>MTAQISPTVVDAVVIGAGFGGIYAVHKLHNEQGLTVVGFDKADGPGGTWYWNRYPGALSDTESHLYRFSFDRDLLQDGTWKTTYITQPEILEYLESVVDRFDLRRHFRFGTEVTSAIYLEDENLWEVSTDKGEVYRAKYVVNAVGLLSAINFPDLPGLDTFEGETIHTAAWPEGKNLAGKRVGVIGTGSTGQQVITALAPEVEHLTVFVRTPQYSVPVGNRPVTKEQIDAIKADYDGIWDSVKKSAVAAGFEESTLPAMSVSEEERNRIFQEAWDHGGGARFMFGTFGDIATDEAANEAAASFIRSKIAEIIEDPETARKLMPTGLYAKRPLCDNGYYEVYNRPNVEAVAIKENPIREVTAKGVVTEDGVLHELDVLVFATGFDAVDGNYRRIEIRGRNGLHINDHWDGQPTSYLGVTTANFPNWFMVLGPNGPATNLPPSIETQVEWISDTVAYAERNEIRAIEPTPEAEEEWTQTCTDIANATLFTRGDSWIFGANVPGKKPSVLFYLG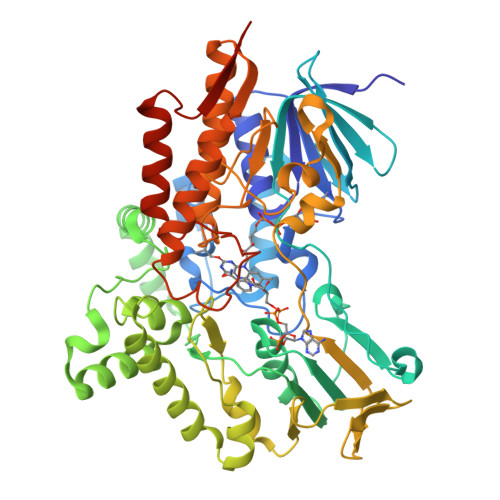GLGNYRNVLAGVVADSYRGFELKSAVPVTALEHHHHHH[2x]>GCUUCGGCN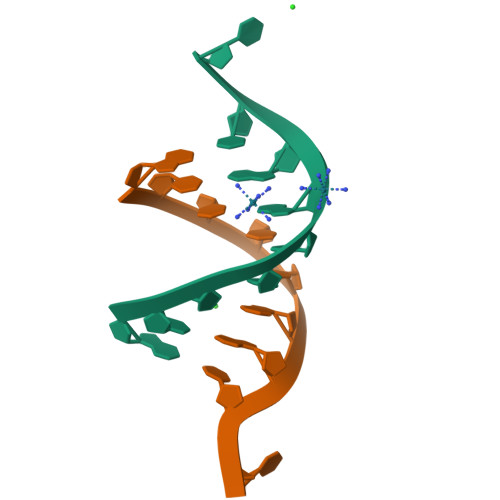[2x]5-METHYL-5H-INDOLO[3,2-B]QUINOLINE | C16 H12 N2 | 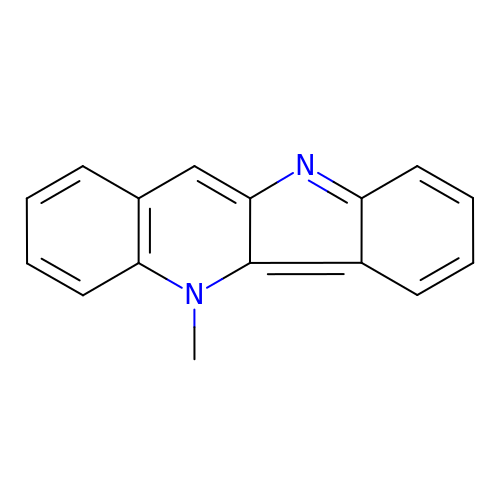KURWKDDWCJELSV-UHFFFAOYSA-N> HNPYYFHEHSFQSRFRSEDGHWRVLERFSQRSDVLRGIENNRFAILEARPQTFIIPHHLDAETVLLVVRGRAAITTVVQERKETKRESYNAERGDVMVIPAGATIYLVNHENEDLQIVKLIQPINNPGEFKDYLSAGGEDQSYYTVFSNDVLEAALDIPRDRLERVFKQHSERRGKIIKGSQEQLKALSQRATSVRKGGRGTRALIKLENQTPVYSNQYGQMFEACPDEFPQLQRTNVA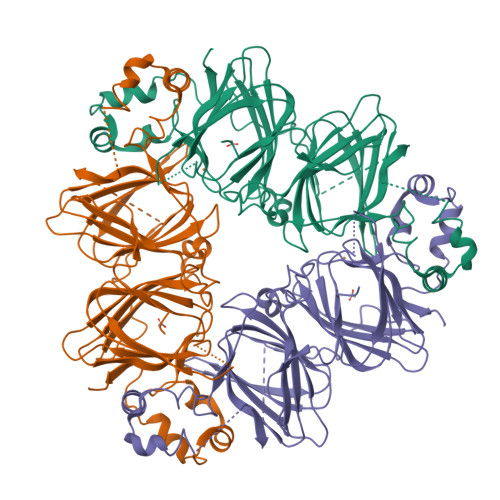AAIVDIKQGGMMVPHFNSRATWAVFVAEGAGSFEMACPHLEESEGRSSRFERVAGHLSPGGLLVVPAGHPIAVMASPKENLRLVGFGINAQNNLRNFLAGKENIMNEVDQEAKELTFNIKGKEADEIFKSQRESFFTKGPVG3,5-DIBROMO-4-(3-ISOPROPYL-PHENOXY)BENZOIC 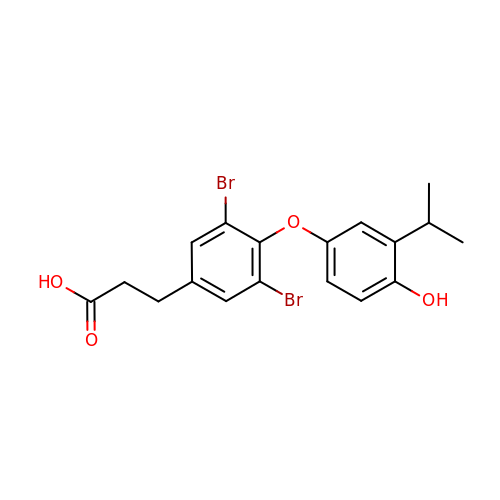ACID | C18 H18 Br2 O4 | DGODJDXDANWOEP-UHFFFAOYSA-N> MSNKEKNASETRKAYTTKMIPRSHDRMKLLGNFMDYLMDGTPIFFELWNQFGGGIDRDIISGTANKDKISDDLLLAVNWFKVMPINSKPQGVSPSNLANLFQQYSGSEPDIQAQEYFASNFDTEKHQWKDMRVEYERLLAELQLSRSDMHHDLKLMYKEKCIGLSLSTAHYITSVMFGTGAKNNRQTKHQFYSKVIQLLEESTQINSVEQLASIILKAGDCDSYRKLRIRCSRKGATPSILKIVQDYELGTNHDDEVNVPSLIANLKEKLGRFEYECEWKCMEKIKAFLASKVGPYYLGSYSAMLENALSPIKGMTTKNCKFVLKQIDAKNDIKYENEPFGKIVEGFFDSPYFESDTNVKWVLHPHHIGESNIKTLWEDLNAIHSKYEEDIASLSEDKKEKRIKVYQGDVCQTINTYCEEVGKEAKTPLVQLLRYLYSRKDDIAVDKIIDGITFLSKKHKVEKQKINPVIQKYPSFNFGNNSKLLGKIISPKDKLKHNLKCNRNQVDNYIWIEIKVLNTKTMRWEKHHYALSSTRFLEEVYYPATSENPPDALAARFRTKTNGYEGKPALSAEQIEQIRSAPVGLRKVKKRQMRLEAARQQNLLPRYTWGKDFNINICKRGNNFEVTLATKVKKKKEKNYKVVLGYDANIVRKNTYAAIEAHANGDGVIDYNDLPVKPIESGFVTVESQVRDKSYDQLSYNGVKLLYCKPHVESRRSFLEKYRNGTMKDNRGNNIQIDFMKDFEAIADDETSLYYFNMKYCKLLQSSIRNHSSQAKEYREEIFELLRDGKLSVLKLSSLSNLSFVMFKVAKSLIGTYFGHLLKKPKNSKSDVKAPPITDEDKQKADPEMFALRLALEEKRLNKVKSKKEVIANKIVAKALELRDKYGPVLIKGENISDTTKKGKKSSTNSFLMDWLARGVANKVKEMVMMHQGLEFVEVNPNFTSHQDPFVHKNPENTFRARYSRCTPSELTEKNRKEILSFLSDKPSKRPTNAYYNEGAMAFLATYGLKKNDVLGVSLEKFKQIMANILHQRSEDQLLFPSRGGMFYLATYKLDADATSVNWNGKQFWVCNADLVAAYNVGLVDIQKDFKKKLEHHHHHH

Cas12i is a newly identified member of the functionally diverse type V CRISPR-Cas effectors. Among them, Cas12i is characterized by a relatively smaller size (1033-1093aa) compared with Cas12a. Cas12i has substantially different efficiencies in cutting two strands of target DNA, which results in a nicking activity that could be utilized to develop a double-nicking approach for genome editing with high specificity. In Cas12i1, the REC lobe consists of the Helical-I domain and the PAM-interacting (PI) domain, whereas the NUC lobe comprises the Wedge (WED), Helical-II, RuvC, and Nuc domains.

The second ternary complex uses the wild-type Cas12i1 to form the R-loop complex after target DNA cleavage (hereafter termed the post-cleavage R-loop complex) and its crystal structure was determined at 2.45 Å resolution. In the post-cleavage R-loop complex, both NTD and TD strands are already cleaved by Cas12i1. The PAM-distal region of the target duplex is released, and the PAM-proximal region of the target duplex is retained in the complex. Interestingly, the cleaved NTD strand stretches out of Cas12i1 and is captured by the neighboring complex from another asymmetric unit. Correspondingly, the cleaved NTD strand of the neighboring complex is determined passing through the RuvC catalytic pocket of the post-cleavage R-loop complex. The overall conformation of the unpaired region dA(6*)–dA(13*) of the NTD strand from the neighboring complex extended into the post-cleavage R-loop complex resembles that of the unpaired region dC(11*)–dC(18*) of the NTD strand in the pre-cleavage R-loop complex. Hence, the post-cleavage R-loop complex not only represents a state of the R-loop complex after the cis-cleavage of the target duplex, but also provides additional information about the pre-cleavage state for the trans-cleavage. For some unknown reason, the cleaved NTD strand accommodated within the RuvC active site was not further trans-processed in the post-cleavage R-loop complex. Notably, three water molecules were identified to form multiple hydrogen bonds within the RuvC catalytic site. Among them, one water molecule interacts with residues D647, N649, D1074 and the phosphate group of dC(11*).>MEQKQRRFTKNIFVLDVTAKTLCGAIAKLSSQPYCQIKIGRVVAFKPVKNPEPKGYVLNVPGPGA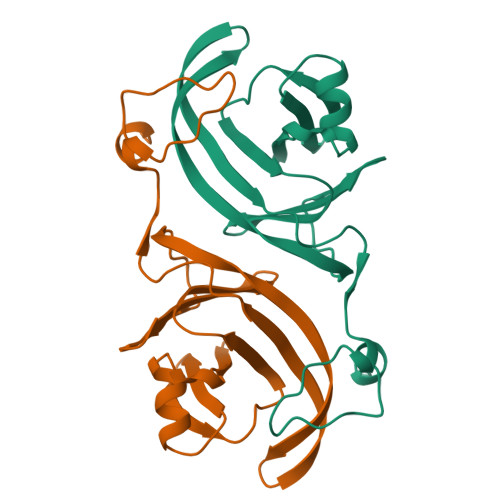YRIQDGQDIISLMLTPHGVEATTERWEEWKFEGVSVTPMATRVQYNGVMVDAEIKYCKGMGIVQPYMRNDFDRNEMPDLPGVMRSNYDIRELRQKIKNERESAPRLQVHSVARPGSENLYPQ[2x]> MTTVLYYLPASPPCRSVLLLAKMIGVELDLKVLNIMEGEQLKPDFVELNPQHCIPTMDDHGLVLWESRVILSYLVSAYGKDE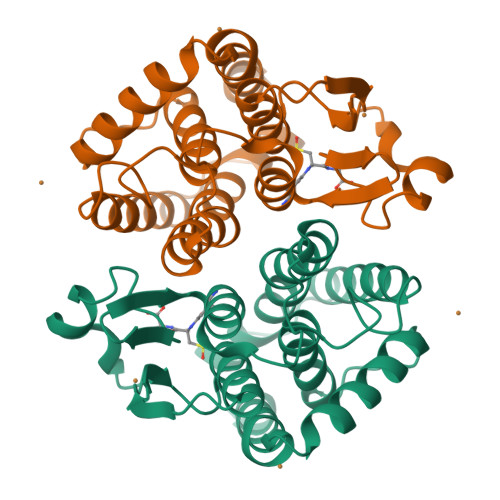NLYPKDFRSRAIVDQRLHFDLGTLYQRVVDYYFPTIHLGAHLDQTKKAKLAEALGWFEAMLKQYQWSAANHFTIADIALCVTVSQIEAFQFDLHPYPRVRAWLLKCKDELEGHGYKEINETGAETLAGLFRSKLKQ Sulfamethoxazole | C10 H11 N3 O3 S | 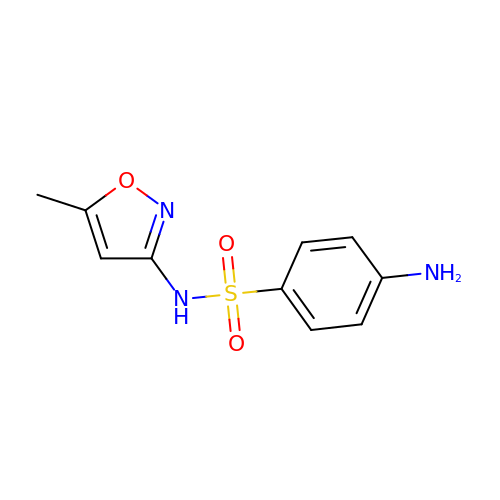JLKIGFTWXXRPMT-UHFFFAOYSA-N> DK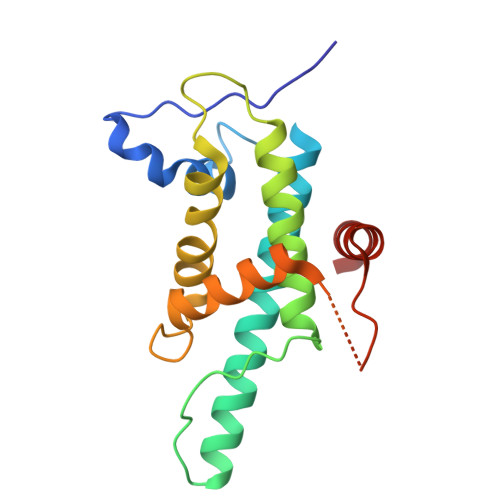EYIPLPPLRDMQDMSKVLFLLSTDKKRYPDGRHRTLDYFRASVEMFVTEVRQEYKRQYQQAQRGGRAMQRFTWKNSGELAICFACCCDNVKLLYDSLQPGPLKPLWDAFVSQLAPMLIIQSRVPEMMLSSQTYHTKYMDWVKGGTRYGGEQSTANVRFPSVADRRVKVETYLRSG>MGSSHHHHHHSSGLVPRGSHMASYALNNNSDFNNGWKFTLSDSVCYSFVNYNPSSWKTVNLPHDWSVDLPFESTAEGCTGFLKGGIGWYSKTFDTPDNFVDKKCYIVFDGVYNNSEYWINGRKLGFHPYGYSPFFYDISDYLNPKGQENRISVRIDHSRYADSRWYTGSGIYRETQLIFTDKLHIPVWGTFVTTPVVSSERATVNIEVRVKNDYSGPRAGEVRTSYFDSKNKKVGEKLTSFLIEAGKEMKINQSVEISNPSLWDVDSPSMYLAKSEILVDGNVVDTKETPFGIRSIKFDAKKGFFLNGKNMKIKGVCLHHDASMIGAALVEDVWRRRLQTLKDGGCNAIRLSHNPGADAFLELCDEMGFLVQEEFFDEWDYPKDKRLNMDEQSIDYITRGYCEYFQEWAERDLKNVMLRSRNHPCIFQWSIGNEIEWTYKGCKESTGFFSADAGGGYFWNQPPYSTQRIREEWAKQPKQTYDIGRTAKKLAAWTREMDTTRPVTANCILPSISYETGYIDALDVAGFSYRRVMYDYAHKNYPDKPAMGTENLGQWHEWKAVIERDYIPGMFIWTGVDYLGEVGTKGREWPQRAIGCGLLDLAGFEKPSFHMMKSLWTDAPFIAIYSQTANKSSYVEKDGKFTDKDPKKPWTQRLWVWEDVNSHWNYTKGEKVVVEIYSNCDEIELFQNGKSLGKRFLKDFEDHIYKWSVDFKDGNIVAKGKKNGKKTTSAIYTTKETNSIKLSVDKVAVDANNTDVIHVTAQLIDRNGRNISWEEKEITFNIGGNYRLLGVENGDHLNVLNYKSNTVKTYKGRALLVLQATDKAGILNINANSGSISSNDLKVEVK[4x]

determined the three-dimensional structures of these four agarases. initiated by GH86 or GH16B, which generates NAOS. depolymerized by GH86, and systematically saccharified by the exo-acting GH117B and GH2C enzymes. exo-acting β-d-galactosidases, while GH117A and GH117B are α-1,3-L-neoagarooligosaccharide hydrolases.

replaced with W657 and C598 in GH2C, respectively. to specifically accommodate the β-linked AHG residue. generate AOS products, which are substrates for GH2C. AOS by GH117B and GH2C, respectively.> MNNSAFTFQTLHPDTIMDA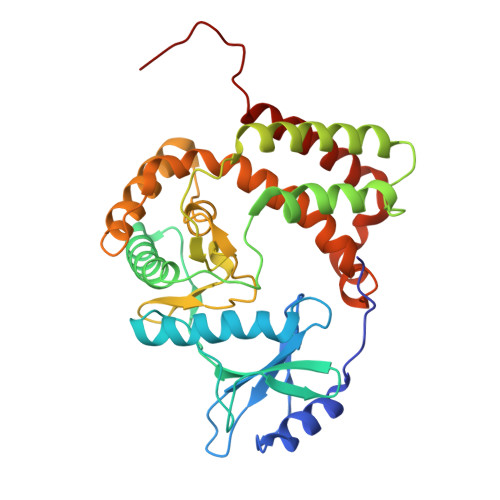LFEHGIRVDSGLTPLNSYENRVYQFQDEDRRRFVVKFYRPERWTADQILEEHQFALQLVNDEVPVAAPVAFNGQTLLNHQGFYFAVFPSVGGRQFEADNIDQMEAVGRYLGRMHQTGRKQLFIHRPTIGLNEYLIEPRKLFEDATLIPSGLKAAFLKATDELIAAVTAHWREDFTVLRLHGDCHAGNILWRDGPMFVDLDDARNGPAVQDLWMLLNGDKAEQRMQLETIIEAYEEFSEFDTAEIGLIEPLRAMRLVYYLAWLMRRWADPAFPKNFPWLTGEDYWLRQTATFIEQAKVLQEPPLQLTPMY> GVKLH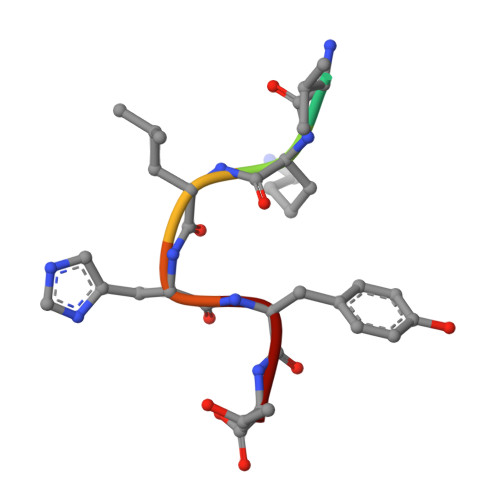YT>SFSVEFKATENEIVSGKLDADTPAFHLVMSDSGEHKGWNVRPTGASEGGQMVSADGTRVDLHTNELSW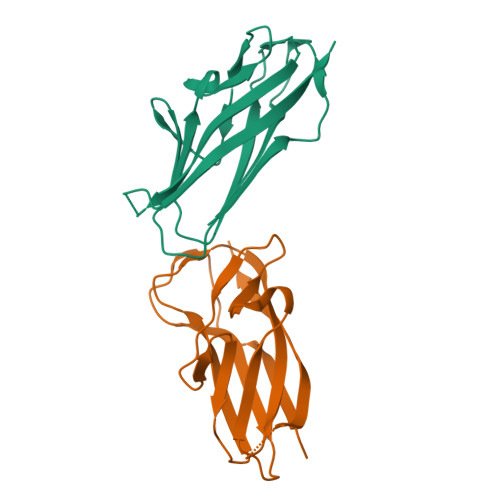DNDHWWIDDGSERVEATFFLAAGDEVKAGEYQFTGRVEEYVEDNKQEPTVINSKDISATKTVKE[2x]> HVKPPQFTWAQWFETQHINMTSQQCTNAMQVINNYQRRCKNQ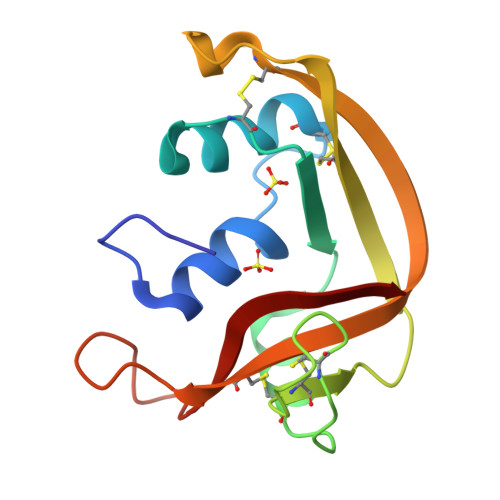NTFLLTTFANVVNVCGNPNMTCPSNKTRKNCHHSGSQVPLIHCNLTTPSPQNISNCRYAQTPANMFYIVACDNRDQRRDPPQYPVVPVHLDRII>MAHHHHHHVDDDDKMTTSPVHEQLQVPQCLAAKITVPHKILAENKEFKIIDVLSSDVETLTILADKVSCGHFVNVSHKLTGTLAANQQQSAQKLLQKKLVKPFGVSKLHKDVYEIKHEEEVNAALKEIVSDNIWQTLTHMTSYYNRSATKDTGVETANWLKSKFEQMAVEYGRTDTSTFFVKTGWYKQPSLVTVIGKDIKAPAIVIGAHMDTLDGRMPGAGDDGSGSSSIMEAARVILSSKTTFKRPIYFIWYAAEERGLVGSQHVVQHFQEQSIPVKAVVQFDMTGYRNDANDPTMWVFTDYTDRDLSNYLAKLIDHYIHVPVDYSRCGYGCSDHASWNEEDIPAAFPCETSFADHNPYIHTSSDKMDLLNLEHMTNFSKLAVAFAIELASE[2x]

LapA is a protease-activated, broad-spectrum aminopeptidase. LapA is annotated as a leucine aminopeptidase, and the Merops database assigns LapA as a member of the M28 family of peptidases (subfamily E). Given the enzymatic activity of LapA, which was revealed by structural analysis, we posited that LapA promotes L. pneumophila growth in A. castellanii by cleaving aminopeptides to release amino acids for uptake by the parasite. Thus, we infer that ProA cleaves and activates LapA.

To confirm the activities of LapA, we purified recombinant LapA-His6-tagged protein containing 378 amino acids of the mature lapA product (minus the 23-residue signal sequence). The structure of LapA contains two molecules in the asymmetrical unit, and all residues could be built except for the N-terminal His tags and residues within the interdomain linkers (residues 82 to 101) that connect the PA domain (residues 1 to 81) and aminopeptidase domains (residues 102 to 378). The PA domain is formed of four helices and three β-strands, and the aminopeptidase domain has nine helices and seven β-strands. Although LapA was purified as a monomer, in our structure, the PA domain of one chain was associated with the aminopeptidase domain of an adjacent chain, which formed a domain-swapped dimer. The domain-swapped monomers were essentially identical, with a root mean square deviation (RMSD) over Cα atoms of 0.083 Å (without linkers), although variations were seen within the interdomain sequence. In our structure of LapA, the PA domain covers the active site and substrate-binding pocket and thus represents the proenzyme form of LapA. The structure of LapA is similar to those of several known aminopeptidases. For example, the positions of active-site residues in LapA and LapB structures are almost identical, while there is a significant reorganization of helices between PA domains. This accommodates differences in their substrate-binding pockets, with LapB’s cavity being wider and more negatively charged, compatible with a preference for positively charged lysine and arginine. The effect of the PA domain is likely due to a transient association between the PA and peptidase domains in LapA, as we observed a monomeric and domain-swapped form in solution.> ETGNSDRYAVYWNRSNPRFHAGAGDDGGGYTVEVSINDYLDIYCPHYGAPLPPA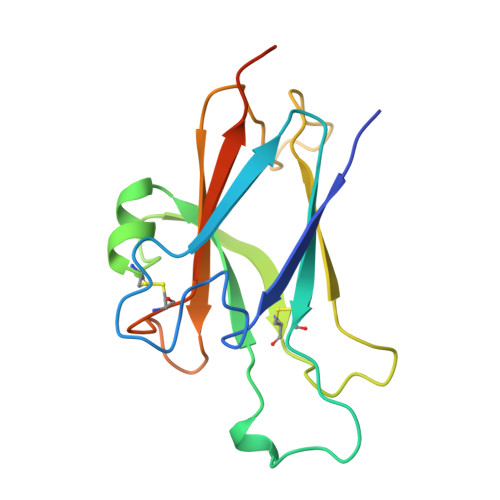ERMEHYVLYMVNGEGHASCDHRQRGFKRWECNRPAAPGGPLKFSEKFQLFTPFSLGFEFRPGHEYYYISATPPNAVDRPCLRLKVYVRPTQETLGTKHHHHHH>[2x]MEELDVDPAETPIPGLGQQNRHIGFSWGPGDLLLYETLYQKQGNSETAARCPFMYLVRSDEDIYSPVLRKLFNESHSIFVGLQKSAEEASGKSRKAQLVQVSRNYRSVLRACMEEMHTLSESTRETAQKYISQISILSAMELSWNLCEILFIESAPAGPLLILLLEWVRLHVCEVDNIVQDVLRSEKPTEHEKFWDGVTGYVLQGRMNEARQLLAKEASTSASARSMCRVLDDLLKKMPMLHTGGTQTLTEFELKWQHWREECERHLQNGTFSSNVHMEAVCRVLLGDEEVLLEKRDLMTTWYHFLVSRLLFKHPTVKPTELHFYAQSSLDMFLAGDSCPEPLDNILLAAFEFDIHQVIKEFSIVSSNWWFVAHLTDLLDHCQLFQAHNLYFGANMREFLLLDYASGLFSHHSLWQLGVDYFDYCPNLGREYLKLHMERIPLSTEKKALKALRICEQRQMTEQVRSICKTMAMQSLCNRRLGSALSWSIRAKDAAFATLISDRFLKEYCERGNFTDLDLIDNLGSAMLLSDRLTFLGKYREFHRMYSQEQFSEAASLLLSLMTARIAPCSFWLTLLLDALPLLEQKQVIFSAEQTYELMRCLEDRMAAKLESTSPDEIQKQDSSIDNTKVEMLRLALARNLARAIVTEGALQE;>[2x]MADKFAAKFVSHKISRTRWRPVSASSLQQPDVFATGSWDNEENKVCVWATSDFGATSLDEEYQGDPKQLCDIKHPGDVMDMQFLDKERIVTGSSTGTVTIFRHHENNQTLSVNQRWEQAHYHVGSNMRAPCTAIVCSSPEIVSVGEDGRINCFRAESRDVLRTIDDADSSTMHGVTFLRTTEILTVNSVGQLKLWDLRKQGNDPTQIFSVTGERVPLHCVDRHPNQQHVVATGGQDGMLCIWDVRHGKMPMSLLNAHEAEMWEVHFHPSNPDHLFTCSEDGSLWHWDASADSEKPTFLLGGRSTFNISRSSIAPPNANQSLACAWLSTDPTKGQLEITNLLPSSTLSVNSLDVLGQNLVCGTDAEAIYVTRRLFS;>MFVARSIAADHKDLIHDVSFDFHGRRMATCSSDQSVKVWDKSENGNWHCTASWKTHSGSVWRVTWAHPEFGQVLASCSFDRTAAVWEEIVGESNDKLRGQSHWVKRTTLVDSRTSVTDVKFAPKHMGLMLATCSADGVVRIYEAPDVMNLSQWSLQHEISCKLSCSCISWNPSSSRAHSPMIAVGSDDSSPNIMGKVQIYEYNENTRKYAKAETLMSVSDPVHDIAFAPNLGRSFHILAVATKDVRIFTMKPLRKELSSSGGVTKFEIHTVAQFDNHNSQVWRVSWNITGTVLASSGDDGTVRLWKANYMDNWKCIGVLKGDGNPVGNSYQGFFGSSVGSAGQSLQNSVNGTPSSGRKHS[2x];>[2x]MAAAESHMTSFQAEDWAGSNILPMVQRAGGSTRGIMAASVNLERSYMELIGAERETSRRNFRDLSLRPDVSLVIGGPKYSDCAGGYCYNESGSLLSATRNRFIHWTSYADTLELVELSLDINLLNNAVRLKILNCSILPGGVHICETQNNIIVLILTNQTVHRLILPHPSRMYRSEIISDSHIQSIFTDIGKTNFHDPNNTYVIPAIPGRAPNSTASTAWLSSDGEALFALPSVSGGILVIKMPPRDMEGLVTIAELKQSSVMQRLLTGWMPSSIRGDPGPAHLPVSLAVHTLDHDSYLFALCQDHKLRMWSYKDQMCLMVADMLEYVPVSKDIRQTAGTGHKLRLAYSDTLEILYLGVYLHTPRQGQFCVFQLVCTESNRYSLEHTSSIFTNQETLIDFTFTLSSMNIWALWLDDDNQTVMKHINFERNQAGHWNPVFVNPLPDDDLAIGDEQEPQEAYLECLFAPGRFTIAALQKAIQILRKGSGRVLDLSWEELKKEVTLTVEKEIQNAVVDYDVSQEEFRQINIENWCKFYTCCLQYQETLSRPLALVVHPNTNMVCLLRKGFLSFLAPCSSVEHLYLVPGEHLLTVDESVICDDVDGASDIVSLIQCLHMIADYITEDMAYQMESACCHPQSPERVAEQILEDLIANDIDNIMENIQNKLQDIRNPIQAISFLLQNMDYETNMDMEQSQHNVRLNLSTLYGSVTASSVVCQAIYKISATRFLICRDLLILQHLLLRLGDMALVGAGQLLHSQQELIPRAAQLLLSYYMIRWGSQCLACAVPVDLLESNLQHLSVLELSDSQVEKRRYTSGIQTIVELFFEDVGRKHFPQVFAHLFIQSGSSQVHRSLNWADLIHRITSYLLQLLWPSNPNFQFAECLMRNCQYTQLQEYVRLLLPWCQVNVGSCHFMLAQCYLVAGEGHKALDCFSQAASEVEREDFLEKLIRVEEGESVSPRLQYYNRVLRLLEDVGLPELVIQLATIAISEASDDWRSQAALRTRIFKHHLDMGHNSQAYDALTQIPDTSRQLDCLRQLVVVLCERSQLQDLVEFPYVNLHNEVVGIIESRARAVDLMTHNYYELLYAFHIYRHNYRKAGTVMFEYGMRLGREVRTLRGLQKQVNSYLACLNCLRLIRPEYAWIVQPVSGAVYERPGASPKRNYDGESSAVPSSSQIEILELRDLEKEYVLAQTRLTLAKHNPSTAAIAGSSAAEEMVALLVQAGLFDTAISLCQTFKLGLTSIFEGLACKCIRLQQGGEAAQAEAWEWLAANQLATVITTKESSATDEAWRLMISYLDKYESKNTLYHHCIINKLLSHGVPLPNWLINRYKAMDAAELLRLYLKYDLLEEAAELVLEYVDALLGKGHQYFGIQAPLSATSQLVWFPYSAIDHLRLALGENENNQHNQAILGKLQRKMDEYFQKLKKATDDYKKIVQKPVRA;>[2x]MKQDSASNATYTVDCEDYVHVVEFNPFDSGEAGSLLAYGGISYVVIASCRFQEEDSTVEGIEFKTLKTFHHGERVVAIAWSPETRCDALLPLLRFATAAGDKKIRIFTSDFQDKNEYKVIEGHSGYINDLVFCSPEGTDIASVGDDHTCRIWDLDGKQIAMFILRSPGMSVAWHPEGAFKLMVAEKTGTIRFYDLTTHQAILSLESVQVPLMSADWCVRNTLRIGAVAGNDWIIWEMPRSSYPQDNKPAHADRARMFRWSKCNENVFATTGYPGKMKSQIAIHHLAHPQPILIGTAPVGSGLSWHRRLPLCVVGGYRKLFFWLTEM;>SKYGLQDSDEEDDQLNSAEAKKLKTAPVPPQGKQPPLQQATLPGKVTPPPQSPAVDQLDRVMELDSDMADITQDQDLDSVAEEQDISEEQEPLSASSHIASSLGINPHALQVMKASLLLEEEDGEIMSRFSSFPSSMDPYPDVRSPRLFPSSHAKRPSSIGLLQSKFSAPSMSRLSETVQGSHSPKIHPAAPWSVPAPLAPSFIMPGPAPDTHLRTVGTRRQQELVPLEKSVTHGRGTLMIDMGLFMGRSFRVGWGPNWTLVHNGDKLSERLNAEEDRDMDTIDYGFLPKPTSAKSLTESPFKVHVEKLSLEQKTKDLQSYLLPLEIELKNSTVDKSGPCPHFRPNPGVTAIHDYAGWVRNFSSEAAEVEAVVKQWGLTWTLCESLWGQLKELEASLDEPNEYVKNLERRKAFSHWLAQTAQERIEEEVSLYGPERHIEAVFSYLTGGRISDACRLAQKSGDHRLSLLLSQMVGSQEVRDLITLQLVDWNKLQVDHYIQEERLRVFCLLSGTPVWRSSDNRSINVCSQLDWKRTLGIHLWYMLPPTATVAQALHMYEQAFQEQEGGEPYACYPLPPYLEDCGFSFGDDPSAKFISLQRDVCVHLLKLYSERQYDLCQLLDPSSATPDPLDYRLSWHMWMVLQALNYTHLSGHRQGMLHASYAAQLENVGLWEWAIFVLLHIQDPHVREAAVRELLNRHCVVHDSPESLAKENFLIQRLCLPAQWIHKAKAVRSRRDGDKHKEALYLLKSHQWNQCHKLVTRHLAADAVINENYRYLRGFLGELARPEHCKHIQDWETAGKVYLDYISVIEMLNQIRQDECSGGELEKLHTKVMSLCKWVELIQCYSAKGRLAQSEMAKRVANILRVVLSLQQPPESMSDSSSEPRVPLRLLAPHIGRLPMPEDYALEELRGLTQSYLRELICGS[2x];>[2x]MVSVINTVDTSHEDMIHDAQMDYYGIRLATCSSDRSVKIFDVKNGGQILIADLRGHDGPVWQVAWAHPMYGNILASCSYDRKVIIWKEENGTWEKTYEYTGHDSSVNSVCWAPHDFGLVLACGSSDGAISILTFTGDGPWEVKKISNAHTIGCNAVSWAPSVIPGSLVDQPSSQKPNYIKRFVSGGCDNLVKIWREEDGQWKEDQKLEAHSDWVRDVAWAPSIGLPTSTIASCSQDGRVYIWTSDDAATNCWTPKLLHKFNDVVWHVSWSITANILAVSGGDNKVTLWKESVDGQWACISDVNKGQGAVSTVTEGQLNDQ;>[2x]MDMLSPVVREAEVSRAARRQSSNRKNPADESWSNATPTRGPSSRTTGQTLFRQHMTPQTWNSSRPPDVSAILGTVGRSPRLLQTPGRLANLSMMSNPDDSVWTTTFSPGRTGMYTTLDSPSFTEDITLSAVMLQEEDPGEAATMSMYPDFLKSFLEHPSSAVFELIEQYEATCNTQITLLKKIVKRVTPGQQKFSKTASILWLLQQEMVTWRLIAALYRDRIQSALEEENMFEIAAPNASEKTIVDKLFQRDTLVRQSQLVVDWLESIAKDEVGDFSDNIEYYAKSVYWENTLHTLKQRSMLSLGSSRPLVSELDPDAPIRQKLPLDDLDREDDIRLLKYLFTLIRAGMTDEAQRLCKRCGQAWRAATLEGWKLYHDANINGGTELQAVEGNPYRCVWKTCCWRMAEDEQFNKYERAIYATLSGNLKQLLPVCESWEDTVWAHFKVMVDSLVEQEIRASIISFNEANELPREYLEANWTLDSVFEELQATDKKRVLEENREHYHIIQKFVILADVDGLMDEFSEWLSNGKNLLLGHLLRFMTHLLLFFRTLGLQAKEEVSVEVLKTYIQRLINEKQIELIAFYVSHLPQELAISQYAVFLENITDPDQRQRCLELAKEAGLDVASITKTVVENTRKKDAGEFAHHDFAPALDSGTSEEDRAKIDVIDWLVFDPAQRAEALKQSNAIMRKFLASKKHEAAKEVFAKIPQDSIAEIYSQWEEQAMDSALPAEDDNAIREHLCIRAYLESHEAFNEWFKHINSPPQKPTLVGQASFTEKVAHEHKEKKYEMDFGIWKGHLDALTSDVKEKIYNVLLFVDGGWMVDVREDTEEDPERSHQMVLLRRLCLPMMCFLLHTVLHNTKQYKDCLRLADIVSSENQKLYTVFSKTEMRNLLQKLRESSLMLLDLQLDPLGYEIQS;>MFPSPRAQGMGSARRPFNSRLTGGRKALGPGVTASSSPSALYSPVGRRVSASGARSTPSRVYLHPAASETVNYNVQLFGSSLPVKVMEALSNASADEPMAACIHEGGWAWLACNDRLIIWKISHSSSAKLMVCKELPLPLSDSEWSADLVDICAQTGDPAAAQSVALMAATPEGSSRYWPNILHEGTYIESYTEFGSSLCAFVTAVKGNSFILSSEKNQLVRLTPDASGKMNQRVLPQGQGMLSGIGRRVSTLFGILSPAVESTLCSVLWDKGDCFYTLTDSSINKWDLDDTSESQVLNWDMSRVLREYISDAIWGSESDYDDIKAGININYLSLNQNCDGLVILSAAWHPGD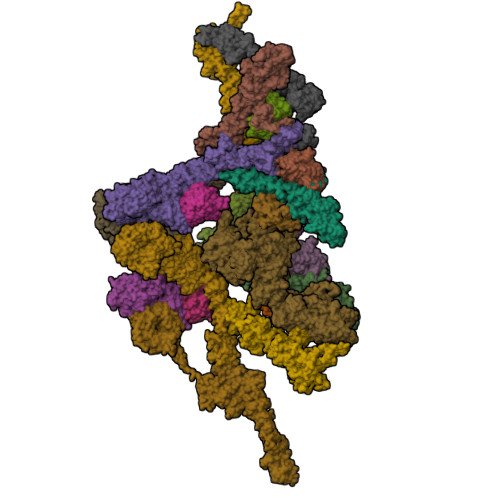NPCQIYYTLVTVKDEGYNISDEITVEVTQFNPVFQARGMQLCQLVVPNFSSQACYLYTQEMIFACSTGTGRSTLPQEKIPFEAQGDNIVGAGSCEGWPVFFIRKSGMLTVVARETASVLPEHMEESLSSVSKSSRQAVVKDSRPDQIAHDDKTKHLKAAFLRYCRKDILGAQSMVDSLFSDSDMEPDDELDLAVNQISVDLIDDYPASDPRWAESVPEEAAGFSNTSLILLHQLEDKMKAHSFFVDFLHQVGLFSRLSTCQTKGMLVATRLLLSEHAEKLSAAIVLKNHHAKLPVLVNSAIQLALDKRMCTVPQNLTAADVYFREVSQMEIIFECLVDKEEADLESTSIDSVEWANIVVNVNTILKDMLHVACQYRQSKNSLYKNESGIQEPEHVPWTASSGTAGIRSVVTRQHGIILKVYPQADSGLRTILIEQLAALLNYLLDDYVTQLKSIDKLANEERYNILEMEYAQKRSELLSPLLILGQYAWASNLAEKYCDFDILVQICEMTDNQSRLQRYMTLFAEQNFSDFLFRWYLEKGKRGKLLSQPASQHGQLAAFLQAHDHLSWLHELNSQEFEKAHRTLQTLANMETRYFCKKKTLLGLSKLAALASDFQEDVLQEKVEEIAEQEHFLLHQETLPKKLLEEKQLDLNAMPVLAPFQLIQLYVCEENKRANENDFMKALDLLEYIGDDSEVDVEELKLEILCKAIKRDEWSATDGKDDPIEATKDSIFVKVLQNLLNKGIELKGYLPKAETLLQSEELNSLKTNSYFEFSLKANYECYMKMQS[2x];> MAAQLALNSEASLWGPYREIWQTVLSALIKRQPEAVHSLDIVLKKYKPDFISLFKNPPKSAQQHERVQKASTEGIPIKGTQRTRILEEQLIKEAFILSDLYNIGEIAAVELLLIGEQQQPTFHGLTRGLVAILLYWDGKSCMAESLLHLIQARKGKTFTLDHSPEVVSMVTRFTDDLMEQGLTNKILTLISQIDVNNEFDKLKKERGLGNKKHRKEVSDLIKECQQSLAHSLYSWSCQTPLNREDTLLLIGYLEKVTVEGDGSLDKVNLTLLMSLLYCLDVGFLEQGTDDREELMKQASMFMDRQYIAAIHNRLQNTQPWKSPGMQATVRLAWALALRGISQFSEVLEFSEADEPMAEIAIGGNVFLFLTEAVVGSESFCTDEFFIRRIHKLVTDFPTLMPMKVKQLRNRAEEDARLIQMSMQMGNEPPASLRRDLEHLLLLIGELYRKDPFHLELALEYWCPTEPLQSTSLMGSFLGVAHQRPPQRQVLLSKFVRQMSDLLPATLYLPYLKMLRGLASGPQCAHYCFSLLKANGGSSAENLQAAGGSPVSWDHFFHSLMLYHEHLRRDLPNTDNIHQRHPPLRGITQRELDGLIACLQLTCTIIDWSESARLALCEHAQWMPVVVILGLLQCSIPPLLKAELLKTLAAFGKSPEIAASLWQSLEYTQILQTVRATGLRQGVGIEVELNEIESRCEEYPLTRAFCQLISTLVESSFPTNLGAGLRAPGFEPYLQFLRDTVFLRYRTRAYRRAAEKWEVAEAVLDVFYKLLKDYEPQPEDFVDQYVELQGEERVAFKPPGFSLMHHLLNESPMLELCLSLMEEGVTQLDTYAPFPGKKHLEKAVAYCFMLLNLTLQKENRFMDLLRESHLSMIVTPLEQLLQGINPRSKKADNVVNIARYLCHGNSNAELAFESAKILCSISCNSKIQEKIVGDFTQDQNVSQKLMVGFVSCLDSEEAEELLDSEKEAEDQVKQTNIRYMTKIHILNLLITSLEMKAPNLAMFLLGYELKKPVSTTNLQDSGVLGCPRTCLHSILDILRKGTDVRAGPVAVWDTPHLAELCYQVIYQLCACADTSGPTMRYLRTSQDFLFSQLQHLPFSVEESEISAMNQMSWLMKTATIELRITSLNRQRSHTQRLLHLLLDDMPTRPYSADGEGGMEDESRSLSGFLHFDTTSKVRRKILRILDSIQFSNEIPEPLQLDFFDRSQIEQVIANCEHKNRRGQTVCNVKLLHRVLVAEVNALQGMAAIGQRPLLMEEINTILQYVVERNKLLQCLHAKRHALESWRQLVEIILTACPQDLIPTEHRQLIIRDLLQDLHVKILDDDAAQELMPIVAGAVFTLTAHLSQSVRTELKQPMTASGLGQSQYVQMLDGSFAAPPGTENISAGFASIGDSSLHMILRNLLEFILKTGGGFQRVRAHLYGSLLYYLQIAQRPDEPDTLESAHKSMWERLTAPEDVFSKLQRDNLSIFESYGTALMEVVCRDACDGHDIGRMLALALLDRIVSVDRQQQWLLYLSNSGYLKVLVDSLAEDDVVLRNLLTPQPPLLKALYIYESKMAFLTRVAKSSQGAIELLRSGVIVRLAQCQVYDMRPETDPHGVFGMRETPVFIPAPVERYRQILLPALQICQLILTSSTAQHLQAAGQVLQFLVAHSDTIQAILRSQEGSLGSLQELALLTGIISKAALPGVLNELDIGLNDGSMMELQGHIGRFQRQCLALLNRFGGSDRLRQLSLQDDSSRLDGVSKKDDMELAMQQICSNVMEYCQALMIQNSPSFQQTVCLFTPSLKESASRDGTRQDSQVSILPSWRLPSLGVVIHLLKQSANNFFTYYDIHRQSVGKLQNVEQLPPDEIKELCQSEMPVGADKISTTQKYGLARRRLVKLINSRAKLLSLCSYIIETCLYILWRHLEYYLLHCTTSDSQDPVFSNMTFGNRRFQDTFNTDPNMDPRNLRQNKVSQQDVDTLLREGANSFGESLQKRLLDIESLYCKVRSRHSFIQALVRRIRGLLRVSRV;> MQNLEAQVTGSLVAFPDVTQKALKEDEINLDSVLRGKFSTGRTSLAWLACGPQLEITNSVTGERISAYHFSGLTERPPVVVAVKEFTWQKKTGLLVGLVEAEGSVLCLYDIGISKVVKAVVLPGSVTAVEPIINHGGASASTQHLHQSLRWFFGVTAVVTDVGHVLLIDLCLDEVSSNQDELDASDLEVMSVIPTKIPKLREAATRERRHLCLQLAAPTGTTVSCLSYISRTNQLAVGYSDGYFSLWNMKTLRRDYHVQIEGGRVPVCAVAFQEPENDPRNCCYLWAVQSSESGGDVSLHLLQLAFSDRKCLASGQIMYELLEYCEERYSLDLSGSTLSLRGQSNNTKLLGCQTIEKFRVHGEREDGVHEVTSPDTSVSVFSWQVNTYGQGKPSVYLGVFDINRWYQAQMPDSLRSGQFLRNCSYFAFWSLEAVVNITTQDIIFDILVHERSLSRGIPPSYPPPEQFYYPSTYNFDATCLLNSGLIHFACTGFQKETLHFLKKSGSSLNEAIPDGYNRCLAAGLLAPKFTDVQASSLSQEEQLQAILAAAVETSSLGLLTSCIKRWTAEEQPRSAANLRFVLEWTWKKVTLTKQEFDRLCFRLFDGSCNFIDPHTLQSLQQCHLYFSNLTAVLNCFIAQAKEVTQQGAVDLTNKQSVTRLLTLYASVVLWFCRSGMLPDSSDETVQLTRPFYNYQVIQQYYSDQRKKLERLARGKWDTSSLMIDGLINQFGDRIQQLWSRDDNGTGKYPPANLHALLDVYLLENADEMSKHAITIYFLLDIMYSFPDKPDSSIESFPTAFFVPGSLIKLIQGFWLLDHNDYQNSVDCILNPASSRVMSWQHSQIIENLLCHGDSRQALRYLQVMKPVATTSKEVKLHMTVLLANRSILEAWNLQRLHSSRLNVEELLKHMYEMCQEMGLIEELLKLTFTDFEQGYLHKFLQTTGVQNQELLLVHHLQRANYISALQLNQSLKTNHLNDCDRRLRERSGARNAILDQYGKILPRVQRTLASERAKPYSLPSLVWREVARPKPLSTTAKQAAPGSIITKANFICNVLSKIKEVSTANEKREEYSPYQSMVSEEPTAPPLQDIDVPDAFFGTPINKSRRVSRLLDSVVHPVLMEPTPLTSSDTDNNQTPHKSPLLKTSSPLHSSLRRIAHMRSFAKASEFSLLETPLVVRKAKALAANTASSGYTSITPQSILRSSVRTTPLVSPSVSPGRSLTPPLRPKETKISFMELSFTRHAKAAHSSEGNLLAISPVLRSSPDAVWSVKGKVASFTQNTPVKKLDEIDASSSGIQEESQDEMEVSKEISNISVRSEQASLEYHDAPTPEDLENDEISGTTNSQPQVNEVHHQMEDGQLTEKPAELALTEMQEEFIDSEEREIEYISAPLNGPNALECMTAVPDIYLEDASQCILETPEGSSVSVTGEQECVSSAKDSESVISIHDSDDAHSNLSENDQDSEEIEENNLRVPTTVTRCEEFDLIETKDLEVELEEADSEKTNYKDIYPDATVQLGFTVESIEQRYTCELADRRETPSETDEIEGEHFETENNFSLVLEGDVTEEEILEPSSSKTDLELTRPPIAHQKLISENRENIENCETTEKIPANMSPLVDSDHESKTLETLPSEADLSVAEKVLKGTEEKDVPPEVHSEVVLESKLVGNAMMSLDSSESQEVIISQYDNVISIEKLEMTQEKMYGEKTEQINEGQVSPNRDQSTLVKPLTPRRSIRKSSKPADSSTDIIGNITLPTTPKRGLKKAKENVDTLKNSISVVPEEELTLGTRRITRKATLTALDNPEPLQIKEPPSGEDLQVQPSTPTRGRRGKVITSDDLKEPPSGEDLQVQPSTPTRGRRGRVITSDDLREPPPGEDLQVQPSTPTRGRRGRVITSDDIKESPSVEDLQVQPSTPTRGRRGKVITSDDIKEPPSVEDLQVQPSTPTRGRKGKVITSDDIKEPLSGEDLQVQPSTPTRGRKGKVITSDDIKEPLSEEVLQEQPSTPTRGRRGRVITSDGKGYECVEEKNALPLTPTRITRSKNILEPEKGISQIEPEKGISQIEPDKGLSQIEDTGETEHEVVTPRRGRRGKRVVNELVKHFERNSSQPNIKADTSPPVSPKKVSLRWTRTRSENQRINATEEQASKIQEDLSDTPRKRYKKSSNKMGFEETTDTVTEGAIVEDVQESLIISHLGKNPNTSIVRSARKTALPPVTEDHSEQPLLPPESHSKVHSSLAIADEENKTNTRTRSGNKSSVDVSAITFEFSTPKARTKKTAKGSAVPTELIPSTQYVFSPPSTRTRRATRANVSEAVIEPQLQFQESCEIAETEVPEVPASKPRGRPPKHKAKAVTRVLKKPSWSTPPVEIKLISPPESPAVSETNTKTDSTEAKGAEKISVRRTRRRIIAKPVTRRKMR;> MDGEGFGELLQQAEQLAAETEGVTELPHVERNLQEIQQAGERLRSKTMTRTSQESANVKASVLLGSRGLDISHISQRLESLSAATTFEPLEPVKDTDIQGFLKNEKDNALLSAIEESRKRTFVMAEEYHRESMLVEWEQVKQRVLHTLLASGEDALDFTQESETSYISESGAPGRSSLDNVEMAYARQMYMYNEKVVSGHLQPSLVDLCTEAAERLDDKNVSDLWVMVKQMTDVPLIPASDTLKSRCSGQMQMAFVRQALNYLEQSYKNYTLISVFANLQQAQLGGVPGTYNLVRSFLNIRLPTPIPGLQDGEIEGYPVWALIYYCMRCGDLMAAQQVVNRAQHQLGDFKNCFQEYIHNKDRRLSPTTENKLRLHYRRAVRASTDPYKRAVYCIIGRCDVSDNHSEVADKTEDYLWLKLSQVCFEDEANSSPQDRLTLPQFQKQLFEDYGESHFAVNQQPYLYFQVLFLTAQFEAAIAFLFRLERTRCHAVHVALALFELKLLLKSTGQSAQLLSQEPGEPQGVRRLNFIRLLMLYTRKFEPTDPREALQYFYFLRNEKDNQGESMFLRCVSELVIESREFDMLLGKLEKDGSRKPGAIDKFTRDTKTIINKVASVAENKGLFEEAAKLYDLAKNPDKVLELTNKLLSPVVSQISAPQSNRERLKNMALAIAERYKSQGVSAEKSINSTFYLLLDLITFFDEYHAGHIDLSFDVIERLKLVPLSQDSVEERVAAFRNFSDEIRHNLSEILLATMNILFTQYKRLKGSGPTTLGRPQRVQEDKDSVLRSQARALITFAGMIPYRMSGDTNARLVQMEVLMN> SNAGGSSPITGLVY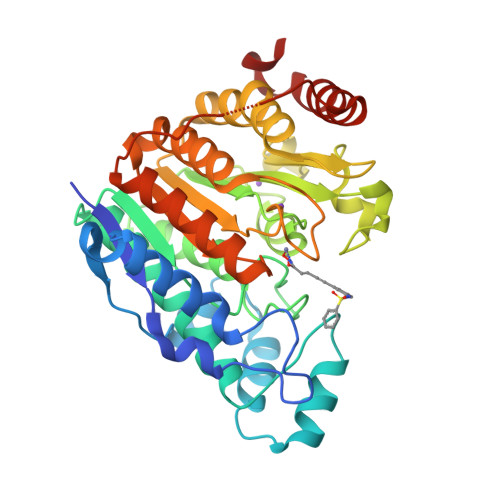DQRMMLHHNMWDSHHPELPQRISRIFSRHEELRLLSRCHRIPARLATEEELALCHSSKHISIIKSSEHMKPRDLNRLGDEYNSIFISNESYTCALLAAGSCFNSAQAILTGQVRNAVAIVRPPGHHAEKDTACGFCFFNTAALTARYAQSITRESLRVLIVDWDVHHGNGTQHIFEEDDSVLYISLHRYEDGAFFPNSEDANYDKVGLGKGRGYNVNIPWNGGKMGDPEYMAAFHHLVMPIAREFAPELVLVSAGFDAARGDPLGGFQVTPEGYAHLTHQLMSLAAGRVLIILEGGYNLTSISESMSMCTSMLLGDSPPSLDHLTPLKTSATVSINNVLRAHAPFWSSLR> MLFLIYRKDRPGSLQVRIDNYAAHLAYLEPLKAKIQVGGPTL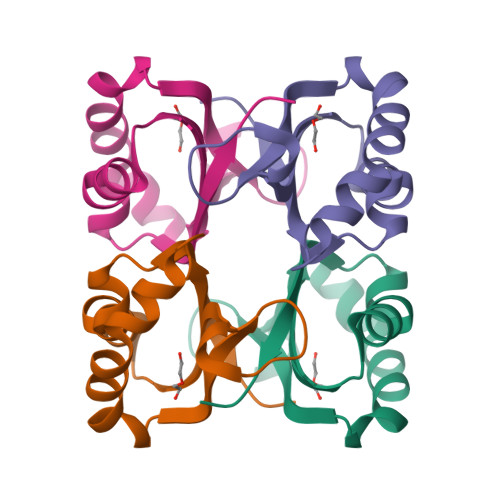GAGTGTDDKDMTGSFLIMEAESWDEVHSFVENDPFTKAGLFAATIVERWKHGKHNDSK> AKLTIESTPFNVAEGKEVLLLAHNLPQNRIGYSWYKG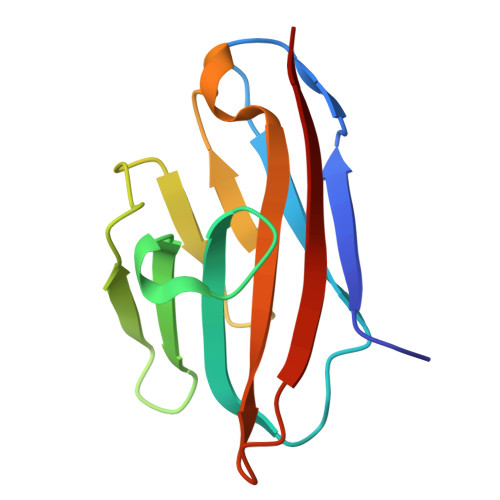ERVDGNSLIVGYVIGTQQATPGPAYSGRETIYPNASLLIQNVTQNDTGFYTLQVIKSDLVNEEATGQFHVY> MACEWLGRYRMISNESLSLLKEMGGKYPEGTKVSFPGRLYNMIDNAKVEDQVKFLVLTLDHIIRLMDAREHMNSVQWNLQTVEHFLTVLNRQSSDLKECVARYQPSHKESYEKKINRHFKILKKNLKKKEYSAQAWEQIRRAVKHHLQRMDIIASIANRR

Teleost type I interferons (IFNs) are categorized into group I and II subgroups that bind to distinct receptors to activate antiviral responses. Based on the patterns of cysteines involved in the formation of disulfide bonds, teleost fish type I IFNs can be classified into two subgroups, one containing two cysteine residues (group I) and one containing four cysteine residues (group II), and can be further divided into seven phylogenetic groups, namely, IFNa–f and IFNh. However, despite a high sequence diversity, all type I IFNs share a similar structure consisting of 6 alpha helices (A–F) that are arranged in unique up-up-down-down topology. Functional studies have shown that CRFB1 pairs with CRFB5 to form a receptor complex that interacts with group I IFNs, while the CRFB2/CRFB5 form a heterodimeric receptor that is activated by group II type I IFNs.

The crystal structure of CiIFNa was determined at 1.58 Å resolution with space group C121 by molecular replacement. As expected, the structure reveals a typical type I ifn architecture of 6 structural elements, denoted A through F. The helices A, C, D, and F form an anti-parallel four-helix bundle, which are arranged in an up-up-down-down orientation. The helix F is straight, which is the hallmark of type I ifn. One disulfide bond formed by Cys3-Cys99 is present in the CiIFNa, linking the N terminal region with helix D, and is analogous to the disulfides found in other vertebrates’ type I ifn. The structure of CiIFNa was compared with that of known type I and III members including human ifn-α2, ifn-β, ifn-w, and ifn-λ and zebrafish IFNφ1 and IFNφ2 by superimposition analysis. It is apparent that CiIFNa has the most structure similarity with zebrafish IFNφ1 (fish group I type I) with an root mean square deviation (RMSD) value of 0.879. Notably, no helix element is present in the AB loop of CiIFNa. The Arg35hIFNw or Arg33hIFNα2 in the AB loop contributes greatly to the interaction with IFNAR2 and is substituted by glycine in the CiIFNa. In the present study, we showed that CiIFNa (group I) interacts with not only CRFB1 and CRFB5 but also CRFB2, indicating that it engages with all three receptors for signaling. Furthermore, mutation of Leu27, Glu103, Lys117, and His165 markedly decreased the phosphorylation of signal transducer and activator of transcription (STAT) 1a induced by CiIFNa in the Epithelioma papulosum cyprini (EPC) cells, and Glu103 was shown to be required for the CiIFNa-activated antiviral activity.> WFEGYDNT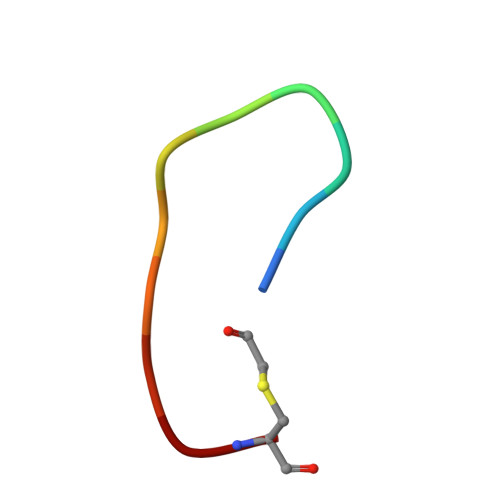FPC>RSWHYVEPKFLNKAFEVALKVQIIAGFDRGLVKWLRVHGRTLSTVQKKALYFVNRRYMQTHWANYMLWINKKIDALGRTPVVG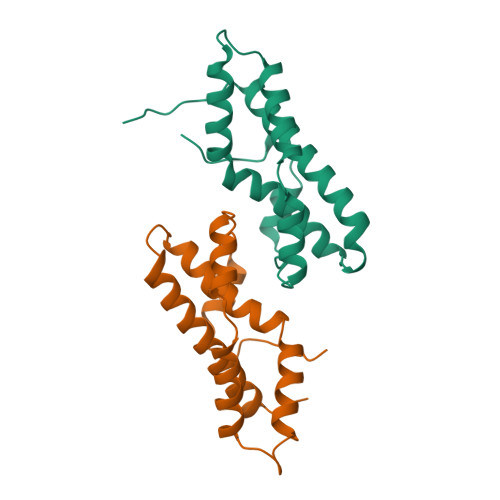DYTRLGAEIGRRIDMAYFYDFLKDKNMIPKYLPYMEEINRMRPADVPVKYMGK[4x]KIF19A, a kinesin-8 sub-family member, is unique in that it possesses both functions, MT-based active motility toward the plus-end and MT depolymerizing activity. We recently reported that KIF19A functions as a MT-depolymerizing kinesin in the control of cilium length. Thus, to elucidate the molecular mechanism of the dual KIF19A functions, we performed crystal structure analysis of the mouse KIF19A motor domain as well as cryo-electron microscopy (cryo-EM) reconstruction of the KIF19A motor domain complexed with a MT. In the catalytic core of KIF19A, the KIF19A-specific feature of adopting two different interfaces for MTs and tubulins is utilized to achieve the dual functions.

Finally, we performed cryo-EM analysis of KIF19A in the nucleotide-free state complexed with a GDP-taxol MT. Cryo-EM reconstruction at a 7.0 Å resolution clarified the interactions between KIF19A specific structures and a straight MT. It should be noted that, presumably because of the weak or unstable interaction between KIF19A and a straight MT, stable and full decoration of KIF19A on the GDP-taxol MT was uncommon; the occupancy of KIF19A is thus lower than that of a tubulin-dimer in our reconstruction. Thus, we finally created an atomic model of KIF19A-free on a MT that has the similar L8 and switch II conformations as KIF5-free and the similar L2 conformation as KIF19A-ADP. The L8 of KIF19A-free on a MT moves to interact with H12 residues of β-tubulin during binding with the MT-lattice and the release of ADP from the catalytic core. This movement is accompanied by approximately 7 degree counter-clockwise rotation of the following helix α3, as also reported in kinesin-13. The switch II α4-L12-α5 of KIF19A-free is retracted to take a similar conformation to that of KIF5-free during MT-lattice binding and ADP release. The length, the location, and the angle of α4 in KIF5-free fit perfectly to the corresponding cryo-EM density of KIF19A-free. This means that KIF19A is able to adjust the switch II conformation to fit the straight tubulin interface on the MT-lattice. When KIF19A is on the MT-lattice, therefore, loop L2 interacts with α-tubulin through the hydrophobic tip and basic cluster, though the acidic cluster will not contribute to the interaction with the MT.

> MKDSGDSKDQQLMVALRVRPISVAELEEGATLIAHKMDEQMVVLMDPMEDPDDILRAHRSREKSYLFDVAFDFTATQEMVYQATTKSLIEGVISGYNATVFAYGPTGCGKTYTMLGTDHEPGIYVRTLNDLFRAIEETSNDMEYEVSMSYLEIYNEMIRDLLNPALGYLELREDSKGVIQVAGITEVSTINAKEIMQLLMKGNRQRTQEPTAANQTSSRSHAVLQVAVRQRSRVKNILQEVRQGRLFMIDLAGSERASQTQNRGQRMKEGAHINRSLLALGNCINALSDKGSNKYINYRDSKLTRLLKDSLGGNSRTVMIAHISPASTAFEESRNTLTYAGRAKNIRTRVKQNHHHHHHH(3Z)-5-chloro-3-[(1-methyl-1H-pyrazol-4-yl)methylidene]-1,3-dihydro-2H-indol-2-one 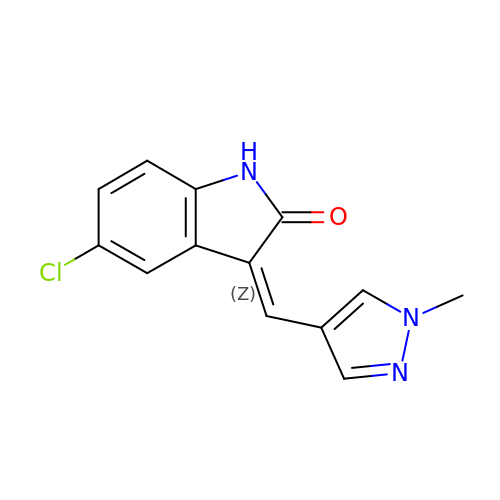| C13 H10 Cl N3 O | XTIZRVLWRIWWNV-WCIBSUBMSA-N>MLPVEGSEEDKSQTGVNRASKGGLIYGNYLHLEKVLNAQELQSETKGNKIHDEHLFIITHQAYELWFKQILWELDSVREIFQNGHVRDERNMLKVVSRMHRVSVILKLLVQQFSILETMTALDFNDFREYLSPASGFQSLQFRLLENKIGVLQNMRVPYNRRHYRDNFKGEENELLLKSEQEKTLLELVEAWLERTPGLEPHGFNFWGKLEKNITRGLEEEFIRIQAKEESEEKEEQVAEFQKQKEVLLSLFDEKRHEHLLSKGERRLSYRALQGALMIYFYREEPRFQVPFQLLTSLMDIDSLMTKWRYNHVCMVHRMLGSKAGTGGSSGYHYLRSTVSDRYKVF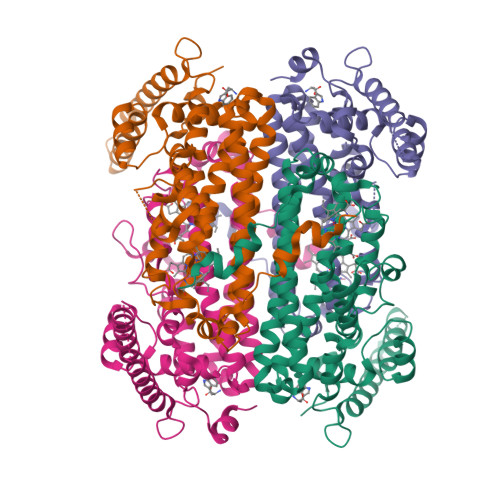VDLFNLSTYLIPRHWIPKMNPTIHKFLEHHHHHH[4x]>[2x]SMEELQNKLEDVVIDRNLLILGKILGEGEFGSVMEGNLKQEDGT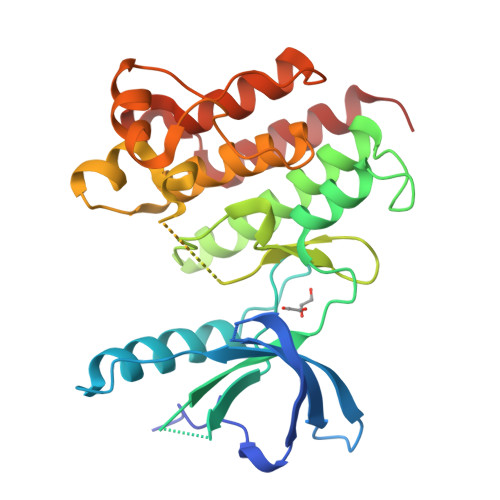SLKVAVKTMKLDNSSQREIEEFLSEAACMKDFSHPNVIRLLGVCIEMSSQGIPKPMVILPFMKYGDLHTYLLYSRLETGPKHIPLQTLLKFMVDIALGMEYLSNRNFLHRDLAARNCMLRDDMTVCVADFGLSKKIYSGDYYRQGRIAKMPVKWIAIESLADRVYTSKSDVWAFGVTMWEIATRGMTPYPGVQNHEMYDYLLHGHRLKQPEDCLDELYEIMYSCWRTDPLDRPTFSVLRLQLEKLLESLPDV> MAIELNVGRKVTVTVPGSSANLGPGFDTLGLALSVYDTVEVEIIPSGLEVEVFGEGQGEVPLDGSHLVVKAIRAGLKAADAEVPGLRVVCHNNIPQSR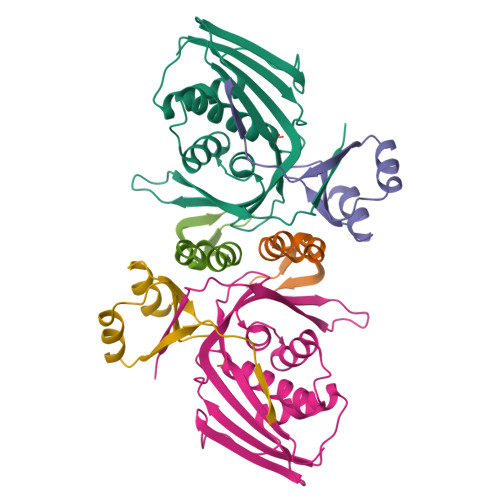GLGSSAAAAVAGVAAANGLADFPLTQEQIVQLSSAFEGHPDNAAASVLGGAVVSWTNLSIDGKSQPQYAAVPLEVQDNIRATALVPN;> FHASTEAVRRVLPTEVTHIDARFNVSRVAVMIVALQQRPDLLWEGTRDRLHQPYR;> AEVLPLTSEWVNRLRNRGYAAYLSGAGPTAMVLSTEPIPDKVLEDARESGIKVLELEVAGPVKVEVNQPHHHHHH>[4x]MAHH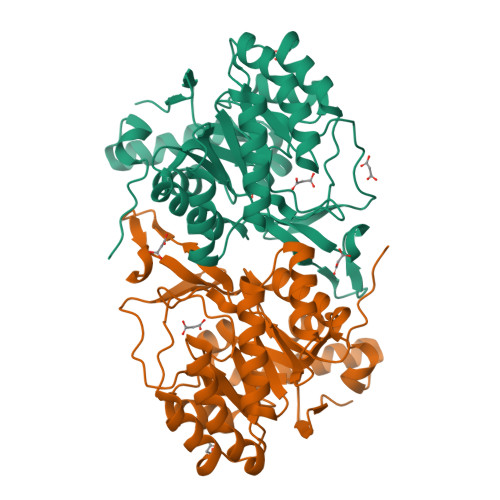HHHHSAALEVLFQGPGSMSLKVNILGHEFSNPFMNAAGVLCTTEEDLRRMTESESGSLIGKSCTLAPRTGNPEPRYFGLPLGSINSMGLPNLGVDFYLSYAAQTHDYSRKPLFLSMSGLSVEESVEMVKKLVPITKEKGTILELNLSCPNVPGKPQVGYDFDTTRTYLQKVSEAYGLPFGVKMPPYFDIAHFDMAAAVLNDFPLVKFITCVNSIGNGLVIDPANETVVIKPKQGFGGLGGKYVLPTALANVNAFFRRCPDKLVFGCGGVYSGEEAFLHILAGASMVQVGTALHDEGPIIFARLNKELQEIMTNKGYKTLDEFRGRVKTMD>[2x]MAVPTGSANLFLRPLILAVLSFLLLSSFVSSVEWLDIDSSDLKALQVIETELGVNSQRSSASDVNPCGRRGVFCERRHSATTGEYVLRVTRLVYRSRSLTGTISPVIGMLSELKELTLSNNQLVNAVPVDILSCKQLEVLDLRKNRFSGQIPGNFSSLSRLRILDLSSNKLSGNLNFLKNLRNLENLSVANNLFSGKIPEQIVSFHNLRFFDFSGNRYLEGPAPVMSSIKLQTSPHQTRHILAETPTSSPTNKPNNSTTSKAPKGAPKPGLELENLYFQGAWSHPQFEKGSHHHHHHHHH

The plant membrane receptor kinase SOBIR1 is a central regulator of plant immunity. It is required for signal transduction of conserved microbe-associated molecular patterns sensed by receptor-like proteins which lack cytoplasmic signalling domains. SOBIR1 and RLPs are likely to form heteromeric signalling complexes. The conserved GxxxG motifs in their transmembrane regions, but neither the SOBIR1 LRR ectodomain nor the kinase domain, are required for this interaction to occur in planta.

Here, we present the crystal structure of the SOBIR1 ectodomain from A. thaliana (AtSOBIR1) and discuss its implications for plant immune signalling. The model was refined against an isomorphous, high-resolution native data set at 1.55 Å resolution. However, both an active kinase domain and the SOBIR1 LRR ectodomain are required for signalling. The crystal structure of the SOBIR1 ectodomain reveals five LRRs sandwiched between unusual N-terminal and C-terminal capping domains. SERK1 shares the number of LRRs and the N-terminal capping domain with SOBIR1, but has a canonical, disulfide-bond-stabilized C-terminal cap. Analysis of the crystal packing with the PISA server revealed a rather small complex interface of ∼1000 Å2 formed by several salt bridges, hydrogen bonds and a few hydrophobic contacts. We next performed analytical size-exclusion chromatography and right-angle light-scattering experiments to assess the oligomeric state of the SOBIR1 extracellular domain in solution.>MAHHHHHHMNPHPVEPRDQIAELLVESPLFSFNCAHFIAFKGFRETLHGHNYNVSLRLRGNIQGDGYVIDFSILKEKVRKV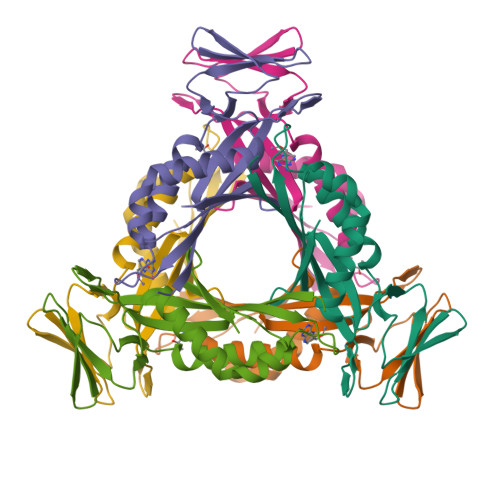CKQLDHHFILPMYSDVLNIQEVNDNFKITCEDNSEYSFPKRDCVQIPIKHSSTEEIGLYILNQLIEEIDLPFLKTRSVNYMEVTVSESPSQKATVHRNI[2x]1-[(3-acetylphenyl)acetyl]-N-(6-bromopyridin-2-yl)-L-prolinamide | C20 H20 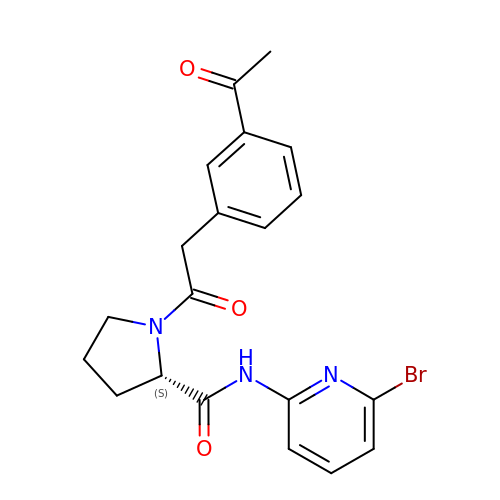Br N3 O3 | QSBZTVCVCZZWLK-INIZCTEOSA-N> GSSHHHHHHSSGLVPRGSMSTSWSDRLQNAADMPANMDKHALKKYRREAYHRVFVNRSLAMEKIKCFGFNMDYTLAVYKSPEYESLGFELTVERLVSIGYPQELLSFAYDSTFPTRGLVFDTLYGNLLKVDAYGNLLVCAHGFNFIRGPETREQYPNKFIQRDDTERFYILNTLFNLPETYLLACLVDFFTNCPRYTSCETGFKDGDLFMSYRSMFQDVRDAVDWVHYKGSLKEKTVENLEKYVVKDGKLPLLLSRMKEVGKVFLATNSDYKYTDKIMTYLFDFPHGPKPGSSHRPWQSYFDLILVDARKPLFFGEGTVLRQVDTKTGKLKIGTYTGPLQHGIVYSGGSSDTICDLLGAKGKDILYIGDHIFGDILKSKKRQGWRTFLVIPELAQELHVWTDKSSLFEELQSLDIFLAELYKHLDSSSNERPDISSIQRRIKKVTHDMDMCYGMMGSLFRSGSRQTLFASQVMRYADLYAASFINLLYYPFSYLFRAAHVLMPHESTVEH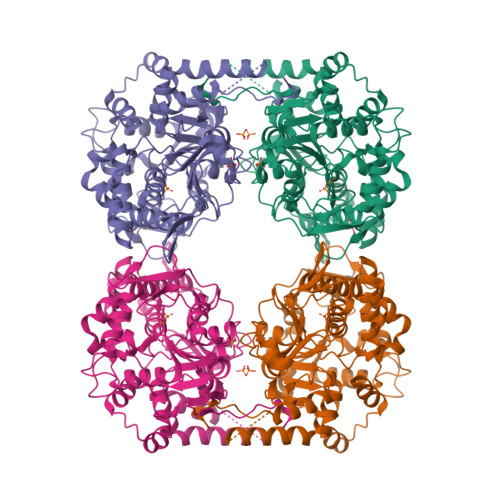THVDINEMESPLATRNRTSVDFKDTDYKRHQLTRSISEIKPPNLFPLAPQEITHCHDEDDDEEEEEEEE Coronaviruses use an RNA-dependent RNA polymerase (RdRp) for the replication and transcription of their RNA genome. RdRp is an important target for the development of antiviral drugs against coronaviruses. Biochemical assays show that the RdRp uses the active form of molnupiravir, β-d-N4-hydroxycytidine (NHC) triphosphate, as a substrate instead of cytidine triphosphate or uridine triphosphate. When the RdRp uses the resulting RNA as a template, NHC directs incorporation of either G or A, leading to mutated RNA products.

To investigate this, we solved two structures of RdRp–RNA complexes that correspond to mutagenesis products after M-templated incorporation of either G or A. We formed RdRp–RNA complexes containing M in the template strand and either G or A at the 3′ end of the product strand. This was predicted to result in the formation of nascent M-G or M-A base pairs in position −1, which is occupied after successful M-templated nucleotide incorporation and RdRp translocation. We indeed obtained RdRp–RNA structures that contained either an M-A or an M-G base pair at position −1. The structures showed an overall resolution of 3.3 Å and 3.2 Å, respectively, with the active center region resolved at ~2.9 Å in both cases. As expected from the scaffold design, the structures showed the post-translocation state with a free NTP-binding site at position +1. The cryo-EM densities at the −1 position of the structures could readily be interpreted by modeling M-A or M-G base pairs. When we interpreted our cryo-EM densities, we assumed that one stable tautomer predominates in each case; that is, the amino-M tautomer forms a base pair with G and the imino-M tautomer forms a base pair with A. These base pairs do not impair RdRp progression, explaining the observed mutagenic pattern seen in in vivo studies of NHC-exposed coronaviruses.

> SADAQSFLNRVCGVSAARLTPCGTGTSTDVVYRAFDIYNDKVAGFAKFLKTNCCRFQEKDEDDNLIDSYFVVKRHTFSNYQHEETIYNLLKDCPAVAKHDFFKFRIDGDMVPHISRQRLTKYTMADLVYALRHFDEGNCDTLKEILVTYNCCDDDYFNKKDWYDFVENPDILRVYANLGERVRQALLKTVQFCDAMRNAGIVGVLTLDNQDLNGNWYDFGDFIQTTPGSGVPVVDSYYSLLMPILTLTRALTAESHVDTDLTKPYIKWDLLKYDFTEERLKLFDRYFKYWDQTYHPNCVNCLDDRCILHCANFNVLFSTVFPPTSFGPLVRKIFVDGVPFVVSTGYHFRELGVVHNQDVNLHSSRLSFKELLVYAADPAMHAASGNLLLDKRTTCFSVAALTNNVAFQTVKPGNFNKDFYDFAVSKGFFKEGSSVELKHFFFAQDGNAAISDYDYYRYNLPTMCDIRQLLFVVEVVDKYFDCYDGGCINANQVIVNNLDKSAGFPFNKWGKARLYYDSMSYEDQDALFAYTKRNVIPTITQMNLKYAISAKNRARTVAGVSICSTMTNRQFHQKLLKSIAATRGATVVIGTSKFYGGWHNMLKTVYSDVENPHLMGWDYPKCDRAMPNMLRIMASLVLARKHTTCCSLSHRFYRLANECAQVLSEMVMCGGSLYVKPGGTSSGDATTAYANSVFNICQAVTANVNALLSTDGNKIADKYVRNLQHRLYECLYRNRDVDTDFVNEFYAYLRKHFSMMILSDDAVVCFNSTYASQGLVASIKNFKSVLYYQNNVFMSEAKCWTETDLTKGPHEFCSQHTMLVKQGDDYVYLPYPDPSRILGAGCFVDDIVKTDGTLMIERFVSLAIDAYPLTKHPNQEYADVFHLYLQYIRKLHDELTGHMLDMYSVMLTNDNTSRYWEPEFYEAMYTPHTVLQ;> MGSSHHHHHHENLYFQSNAAIASEFSSLPSYAAFATAQEAYEQAVANGDSEVVLKKLKKSLNVAKSEFDRDAAMQRKLEKMADQAMTQMYKQARSEDKRAKVTSAMQTMLFTMLRKLDNDALNNIINNARDGCVPLNIIPLTTAAKLMVVIPDYNTYKNTCDGTTFTYASALWEIQQVVDADSKIVQLSEISMDNSPNLAWPLIVTALRANSAVKLQ;> SNASKMSDVKCTSVVLLSVLQQLRVESSSKLWAQCVQLHNDILLAKDTTEAFEKMVSLLSVLLSMQGAVDINKLCEEMLDNRAT> MDQENFHGSSLPQQLQNLHIQPQQASPNPVQTGFAPRRHYNNLVGLGNGNAVSGSPVKGAPLGQRHVKLKKEKISAQVAQLSQPGQLQLSDVGDPALAGGSGLQGGVGLMGVILPSDEALKFVSETDANGLAMKTPVSILQELLSRRGITPGYELVQIEGAIHEPTFRFRVSFKDKDTPFTAMGAGRSKKEAKHAAARALIDKLIGAQLPESPSSSAGPSVTGLTVAGSGGDGNANATGGGDASDKTVGNPIGWLQEMCMQRRWPPPSYETETEVGLPHERLFTIACSILNYREMGKGKSKKIAKRLAAHRMWMRLQETPIDSGKISDSICGELEGEPRSSENYYGELKDISVPTLTTQHSNKVSQFHKTLKNATGKKLLKLQKTCLKNNKIDYIKLLGEIATENQFEVTYVDIEEKTFSGQFQCLVQLSTLPVGVCHG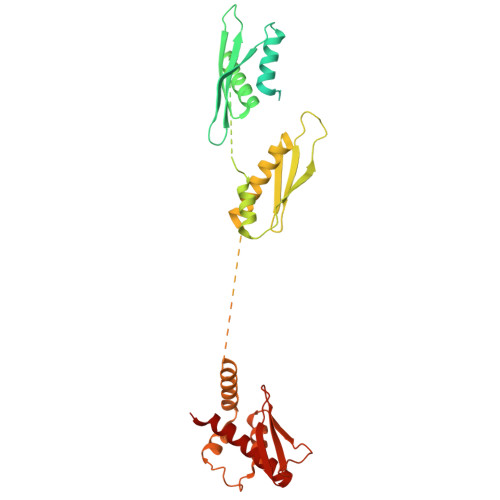SGPTAADAQRHAAQNALEYLKIMTKK>XAVLFVGS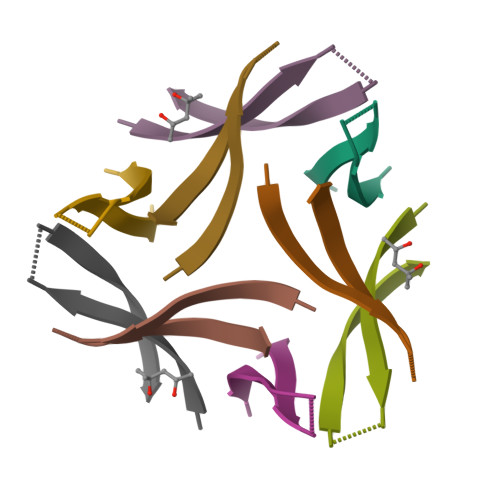XVHGXATV[6x]>[3x]MA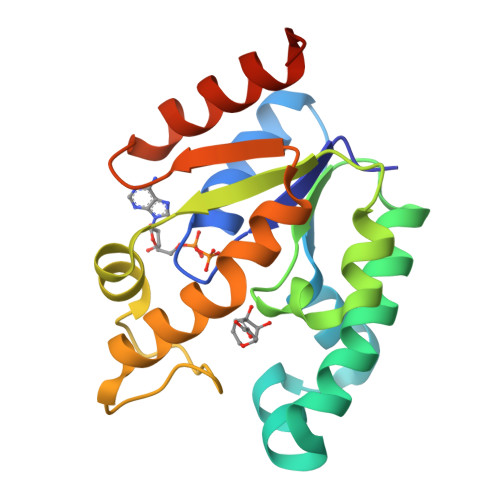PKAVLVGLPGSGKSTIGRRLAKALGVGLLDTDVAIEQRTGRSIADIFATDGEQEFRRIEEDVVRAALADHDGVLSLGGGAVTSPGVRAALAGHTVVYLEISAAEGVRRTGGNTVRPLLAGPDRAEKYRALMAKRAPLYRRVATMRVDTNRRNPGAVVRHILSRLQVPSPSEAAT N-[3-[[(3R)-pyrrolidin-3-yl]oxymethyl]phenyl]thiophene-2-carboximidamide | C16 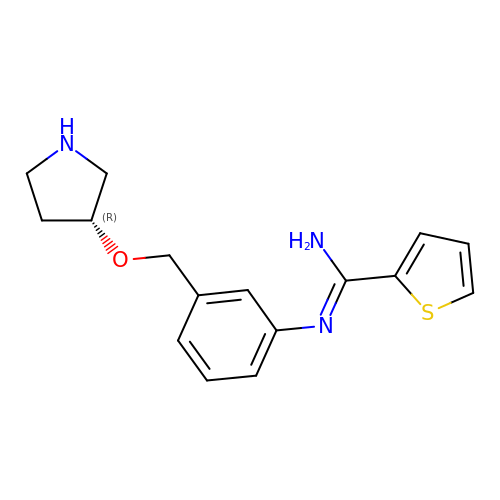H19 N3 O S | OOJUYDKIKUNGMC-CQSZACIVSA-N>MSCINLPTVLPGSPSKTRGQIQVILGPMFSGKSTELMRRVRRFQIAQYKCLVIKYAKDTRYSSSFCTHDRNTMEALPACLLRDVAQEALGVAVIGIDEGQFFPDIVEFCEAMANAGKTVIVAALDGTFQRKPFGAILNLVPLAESVVKLTAVCMECFREAAYTKRLGTEKEVEVI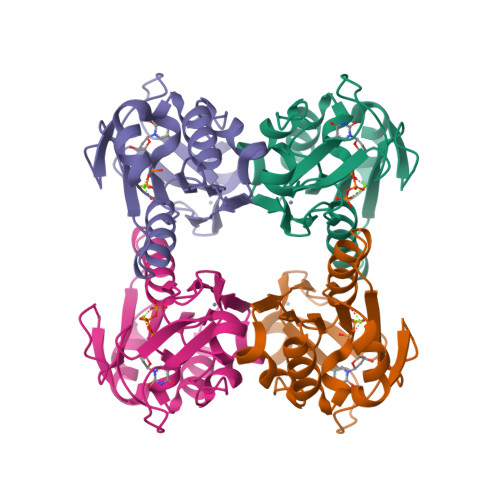GGADKYHSVCRLCYFKKA[8x]> MERYENLFAQLNDRREGAFVPFVTLGDPGIEQSLKIIDTLIDAGADALELGVPFSDPLADGPTIQNANLRAFAAGVTPAQCFEMLALIREKHPTIPIGLLMYANLVFNNGIDAFYARCEQVGVDSVLVADVPVEESAPFRQAALRHNIAPIFICPPNADDDLLRQVASYGRGYTYLLSRSGVTGAENRGALPLHHLIEKLKEYHAAPALQGFGISSPEQVSAAVRAGAAGAISGSAIVKIIEKNLASPKQMLAELRSFVSAMKAASRA;> MTTLLNPYFGEFGGMYVPQILMPALNQLEEAFVRAQKDPEFQAQFADLLKNYAGRPTALTKCQNITAGTRTTLYLKREDLLHGGAHTTNQVLGQALLAKRMGKSEIIAETGAGQHGVASALASALLGLKCRIYMGAKDVERQSPNVFRMRLMGAEVIPVHSGSATLKDACNEALRDWSGSYETAHYMLGTAAGPHPYPTIVREFQRMIGEETKAQILDKEGRLPDAVIACVGGGSNAIGMFADFINDTSVGLIGVEPGGHG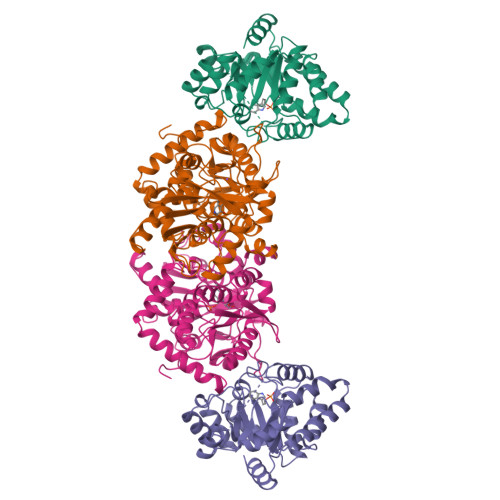IETGEHGAPLKHGRVGIYFGMKAPMMQTADGQIEESYSISAGLDFPSVGPQHAYLNSIGRADYVSITDDEALEAFKTLCRHEGIIPALESSHALAHALKMMREQPEKEQLLVVNLSGRGDKDIFTVHDILKARGLI> GSDELYRQSLEIISRYLREQATGAKDTKPMGRSGATSRKALETLRRVGDGVQRNHETAFQGMLRKLDIKNEDDVKSLSRVMIHVFSDGVTNWGRIVTLISFGAFVAKHLKTINQESCIEPLAESITDV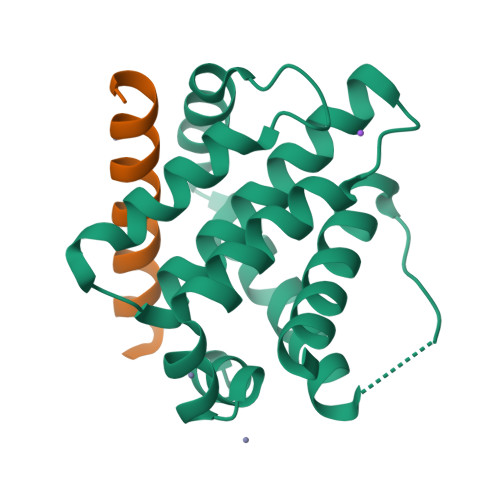LVRTKRDWLVKQRGWDGFVEFFHVEDLEGG;> GGSGRPEIWIAQELRRIGDEFNAYYARRV We look first at the metabotropic glutamate receptor mGluR7, a class C GPCR important for synaptic transmission and neuronal development in the central nervous system. mGluR7 forms a functional dimer with extracellular domains (ECDs) responsible for ligand binding and dimerization (the ECDs in the dimer are disulfide bridged), transmembrane domains (TMDs) that mediate coupling to G-proteins, and short intracellular domains (ICDs) that are largely unstructured. Dimers of mGluR7 have been shown to form immobile clusters at presynaptic sites in neurons and the ECDs have been implicated in this behavior. Thus, the ECD of mGluR7 has been shown to be important for cluster formation in cells. But molecular details of mGluR7 assembly are not known.

To address the mechanisms of assembly, we purified native membrane vesicles (NMVs) derived from cells expressing excess mGluR7. NMVs were generated using N-ethylmaleimide (NEM)/Ca2+ and those containing mGluR7 were enriched using affinity chromatography. mGluR7 clearly forms bulk phase clusters in the NMVs at these high concentrations. Selected proteins within the clusters permit calculation of a cryo-EM density map of an mGluR7 dimer. Using the single molecule translations and angles from image analysis and map refinement to position dimers in the raw images, neighboring pairs of mGluR dimers can be seen to contact each other mainly through the large extracellular ligand binding domains. The contact sites appear multiple, instead of being dominated by a particular pair of surfaces of the ligand binding domains. Micrographs with side views of the mGluR7 bulk phase clusters show strong protein density on the intracellular side of the NMV that does not appear in the final cryo-EM reconstruction of an mGluR7 dimer. While mGluR7 dimers contain only a small number of amino acids on the intracellular side, it is possible that other proteins from the cytoplasm—purified along with the NMVs—could mediate cluster formation. The mGluR7 dimer has twofold symmetry, and the contacts are made through ordered structures on the protein. However, in contrast to HCN1, there appear to be many competing contact surfaces in mGluR7 rather than a dominant favorable surface. Consequently, clusters of mGluR7 are not arrayed with the kind of regularity observed for HCN1.

>MKTIIALSYIFCLVFAGGGGSPSRLEEELRRRLTEPQEMYAPHSIRIEGDVTLGGLFPVHAKGPSGVPCGDIKRENGIHRLEAMLYALDQINSDPNLLPNVTLGARILDTCSRDTYALEQSLTFVQALIQKDTSDVRCTNGEPPVFVKPEKVVGVIGASGSSVSIMVANILRLFQIPQISYASTAPELSDDRRYDFFSRVVPPDSFQAQAMVDIVKALGWNYVSTLASEGSYGEKGVESFTQISKEAGGLCIAQSVRIPQERKDRTIDFDRIIKQLLDTPNSRAVVIFANDEDIKQILAAAKRADQVGHFLWVGSDSWGSKINPLHQHEDIAEGAITIQPKRATVEGFDAYFTSRTLENNRRNVWFAEYWEENFNCKLTISGSKKEDTDRKCTGQERIGKDSNYEQEGKVQFVIDAVYAMAHALHHMNKDLCADYRGVCPEMEQAGGKKLLKYIRNVNFNGSAGTPVMFNKNGDAPGRYDIFQYQTTNTSNPGYRLIGQWTDELQLNIEDMQWGKGVREIPASVCTLPCKPGQRKKTQKGTPCCWTCEPCDGYQYQFDEMTCQHCPYDQRPNENRTGCQDIPIIKLEWHSPWAVIPVFLAMLGIIATIFVMATFIRYNDTPIVRASGRELSYVLLTGIFLCYIITFLMIAKPDVAVCSFRRVFLGLGMCISYAALLTKTYRIYRIFEQGKKSVTAPRLISPTSQLAITSSLISVQLLGVFIWFIVDPPNIIIDYDEHKTMNPEQARGVLKCDITDLQIICSLGYSILLMVTCTVYAFKTRGVPENFNEAKYIGFTMYTTCIVWLAFIPIFFGTAQSAEKLYIQTTTLTISMNLSASVALGMLYMPKVYIIIFHPELNVQKRKRSFKAVVTAATMSSRLSHKPSDRPNGEAKTELCENVDPNSPAAKKKYVSYNNLVI[2x]> RSYGTPELDEDDLEAELDALGDELLADEDSSYLDEAASAPAIPEG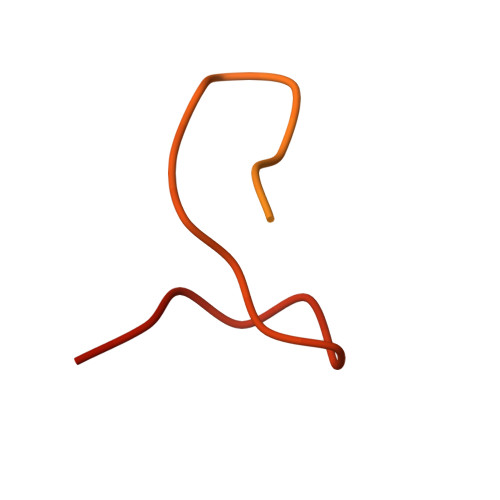VPTDTKNKDGVLVDEFGLPQIPAS> MAKEKKRGFFSWLGFGQKEQTPEKETEVQNEQPVVEEIVQAQEPVKASEQAVEEQPQAHTEAEAETFAADVVEVTEQVAESEKAQPEAEVVAQPEPVVEETPEPVAIEREELPLPEDVNAEAVSPEEWQAEAETVEIVEAAEEEAAKEEITDEELETALAAEAAEEAVMVVPPAEEEQPVEEIAQEQEKPTKEGFFARLKRSLLKTKENLGSGFISLFRGKKIDDDLFEELEEQLLIADVGVETTRKIITNLTEGASRKQLRDAEALYGLLKEEMGEILAKVDEPLNVEGKAPFVILMVGVNGVGKTTTIGKLARQFEQQGKSVMLAAGDTFRAAAVEQLQVWGQRNNIPVIAQ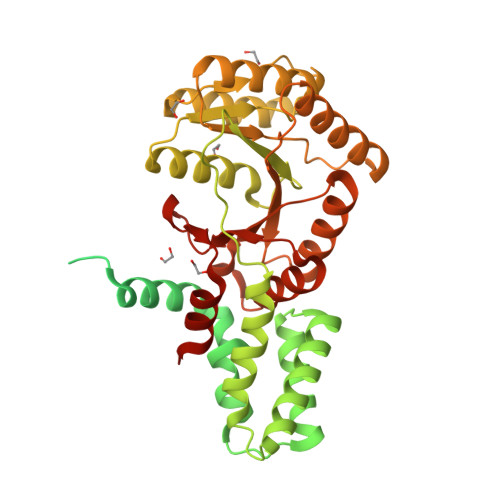HTGADSASVIFDAIQAAKARNIDVLIADTAGRLQNKSHLMEELKKIVRVMKKLDVEAPHEVMLTIDASTGQNAVSQAKLFHEAVGLTGITLTKLDGTAKGGVIFSVADQFGIPIRYIGVGERIEDLRPFKADDFIEALFAREDHHHHHH Aryl-fluorosulfates are mild electrophiles that are very stable in biological media and in vivo and can efficiently react with the side chains of Lys, Tyr, or His residues, when properly juxtaposed by a high-affinity ligand. We report here that a fragment library of aryl-fluorosulfates, when deployed with proper biophysical screening strategies, can identify initial covalent fragments. As a model system to define the most suitable screening approach with our library, we chose the antiapoptotic protein hMcl-1(172–323), given that we recently reported on ligand-first strategies to derive covalent peptide inhibitors targeting active site residues Lys 234, or His 252 with more reactive sulfonyl fluorides, or more recently also His 224 with an aryl-fluorosulfate peptide. The hMcl-1(172–323) construct retained its binding ability for pro-apoptotic proteins and it has been extensively studied to characterize the interaction of hMcl-1 with potential drug candidates. ,,,− Based on our previous experience with covalent agents, we observed that covalent compounds could cause very large denaturation thermal shifts, often with double-digit degrees Celsius, compared to reversible agents.

Finally, the X-ray structure of the complex between fragment hit 2 and hMcl-1(172–323) was also obtained at 1.82 Å resolution, indicating that the compound binds in a deep region within the BH3 binding pocket surrounding His 224. In addition, the contiguous electron density between the compound and His 224 Nε that corresponds to the expected imidazole sulfamate moiety can be clearly observed. Our screening approach resulted in the initial fragment hit 2 whose binding geometry as determined by X-ray crystallography is novel with respect to the several hMcl-1 antagonists reported to date, that almost invariably anchor around an electrostatic interaction with Arg 263 and an acid residue (mimicking a critical Asp acid in the BH3 peptides). The spectral data clearly indicated a large perturbation to the 15Nε and 15Nδ resonances of His 224, compatible with a covalent bond formation at the imidazole ring of His 224. Chemical shift perturbations studies mapping the changes in backbone [15N, 1H] correlations of hMcl-1(172–323) in the presence of fragment hit 2, also revealed that the compound likely binds to the BH3 binding region, closer to His 224 than other binding site nucleophilic residues His 252, or Lys 234. With fragment hit 2, accordingly, which induces the largest ΔT m, hence likely the most effective under the chosen experimental conditions, we observed nearly 100% 1:1 covalent complex formation via MS analysis. Moreover, since reference compound 6 also binds covalently to His 224, we performed a displacement measurement by TSA, and we observed that binding of the covalent hit 2 prevented the binding of the BH3 peptide.

> DELYRQSLEIISRYLREQATGAKDTKPMGRSGATSRKALETLRRVGDGVQRNHETAFQGMLRKLDIKNEDDVKSLSRVMIHVFSDGVTNWGRIVTLISFGAFVAKHLKTINQESCIEPLAESITDVLVRTKRDWLVKQRGWDGFVEFFHVED>MKRVVVTGMAGITSLGETADDIFARFEAGKSGIRYMPEWEQYVDLRTKLAGPVETFHIPKHFNRKVTRGMGRVALMSVVCAETALQNAGLLGHEILSSGEAGVAFGSSAGSVDAVGEFASMLLHQSMSKINATTYIRMMAHTSAVNMTVYFGLKGLTLPTSSACTSGSMAIGQAYEAIKYGKQQVMIAGGAEELSAAGAAVFDVLFATSGMNDQPEKTPRPFDAKRDGLVIGEGAGCLILEEYEHAKARGAHIYAEVIGYGSNTDGQHVTRPESEMMGRCMELALKDASVEAKDIAYVNAHGTS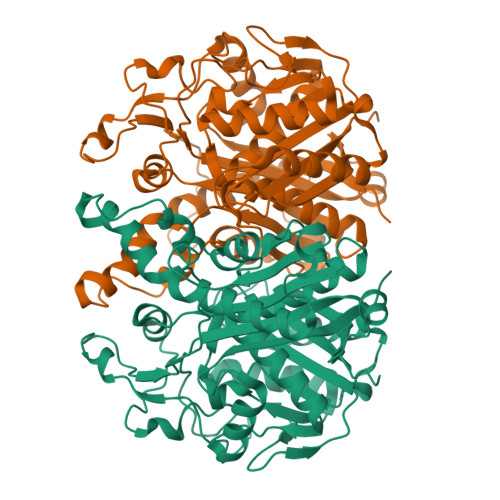TDQGDVAESQATAKVLGYKPISSLKSYFGHTLGACGAIEAWLSIEMMNRGRFIPTLNLDEIDSLCGELDYIVQQPRNLDADIIMSNNFAFGGINTSLIFKRVKQ[4x]> PKPGDIFEVELAKNDNSLGISVTGGVNTSVRHGGIYVKAVIPQGAAESDGRIHKGDRVLAVNGVSLEGATHKQAVETLRNTGQVVHLLLE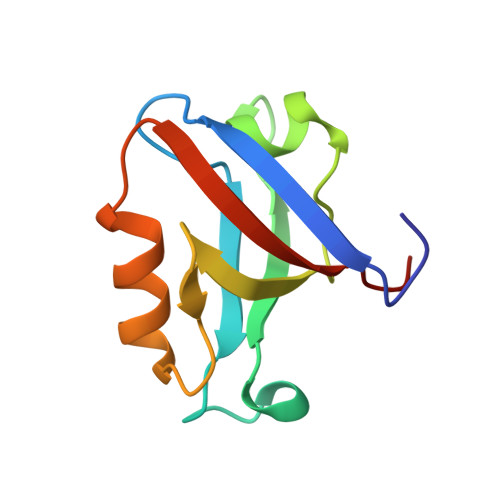KGQSPT>[4x]MAHHHHHHMNDYRIESDLIGELKVPVNAYYGVQTQRAIDNFKISNDHLSDHPEFIKAFAFVKKAAAQTNFELGLLDEIINKNIATACDEIIAGKMHKEFPTDMIQGGAGTSMNMNANEVIANRALELMGHQKGEYQFCSPNDHVNLSQSTNDAYPTAIRIALYNLNKTLVERLELLIQSFRKKADDLKDVIKMGRTQLQDAVPMTMGQEFNAFANTLQEEIARLNTNADLFLETNMGAT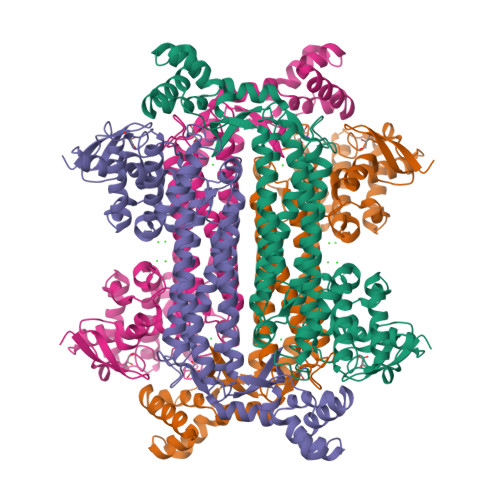AIGTGLNAHPDYAVKCTENLAKISGADVVLASDLVEATPDTGAYVIYSSAMKRMAVKLSKICNDLRLLASGPRAGLYEINLPKMQPGSSIMPGKVNPVIPEVVNQVCFKVIGNDLTVTFAAEAGQLQLNVMEPVLTQSIMESIRFLKNAMDTLREKCIDGITANKEICLNMVKNSIGIVTALNPYIGYKNSTKIAKEALDTGKSVYDLVLEHELLSKEKLDEILAPENMLNPHTKF>MENSKTEQVTGATGITQSTVTAPLPEAVSSLSLAPTVNA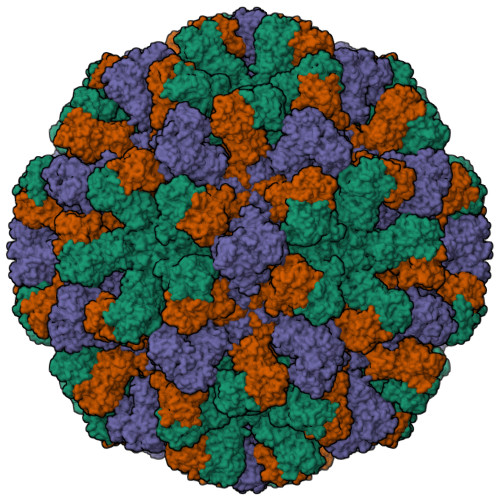LDPWVYLNQTEVPGGTFTVSSATQPGSVLLELEISPELNLYTSHLFRMYAGWSGGFSLKLLVAGNAFSAGKLIAAIIPPNIEVPNSAYLLTGFPHEILDFRTADSMEIIAPDIKNIDYHFRGDKLGKLVVMVYSPLRSTSADFEIEIKLTSAPLPDFKFTMLVPPIQNNALPIWSIPQAPPYSMVNPRSPLTPVVELYINSSYATCNHQLGRYTIYQGAIGNSTFNPSGAWTATCTAEAGSVTGNPNWRYALLDLPDNPTFDPTLPPVPRGFCDWGSGVKSGNKQHLVCFTGKKFAGGFQDVDAHMWDYGDNETVGLDNTYQRTIYISDPSLEKDAQYLVIPMGVSGAANDDTVQVAPNCYGSWDYAPTVAPPLGEQFVWFRSQLPASKTTTTSGVNSVPVNVNALMSPDLIRSAYASGFPLGKVALLDYVLFGGSVVRQFKLYPEGYMTANTTGSNTGFIIPADGYFRFNSWVSPSFMISSVVDLNLQTAVVFR[3x]Given the auxotrophic nature of pneumococci for certain amino acids, the Ami ABC transporter system, orchestrating oligopeptide uptake, becomes indispensable in host compartments lacking amino acids. The system comprises five exposed Oligopeptide Binding Proteins (OBPs) and four proteins building the ABC transporter channel. Crucially, SBPs determine the specificity of their respective transport systems, thereby governing the range of molecules capable of entering the cell. The five lipoproteins exhibit pairwise sequence identity of ~52–60% and share a very similar overall folding.

AliC was also crystallized in the open conformation, and its structure manifests all the characteristics delineated for AliD. Remarkably, the crystal structure of AliC unveils a distinctive three-dimensional domain-swapped dimer arrangement. In this configuration, the Lobe 1 (comprising Domain I and II) of one monomer becomes intertwined with the Lobe 2 (Domain III) of the adjacent monomer, resulting in an overall architecture that is identical for the two functional monomeric units. The resulting entwined dimer adopts an open conformation, but the width of the ligand-binding cleft is expanded compared to that observed in AliD, measuring 29 Å instead of 16 Å. The observed domain swapping in AliC would be compatible with its insertion into the membrane, given that both N-terminal ends would be oriented toward the same side. Nevertheless, to date, there is no supporting evidence indicating that a domain-swapped dimer represents a functional state of these SBPs, including AliC. The domain swap in AliC results in an extended interface area of 5173.1 Å2 [calculated with PDBe PISA v1.52], occurring at a hinge axis passing through the middle of the loop connecting α7 with β14 (residues 290–294), extending between Lobe 1 and Lobe 2. This loop in AliC contains a glycine residue (G290) that is unique compared to other homologs, which typically have a lysine residue at that position (K287 in AliD). For instance, AliD presents a significant number of aromatic residues decorating the binding-site cavity, promoting the binding oligopeptides with a high hydrophobic residue content. Both AliB and AliC share strongly acidic pockets P3 and P4 but AliC features distinctive basic pockets P1 and P2.

> ASKSEKNADAPKTFSYVYAVDPSSLDYSLTSKSSTSDVIGNVVDGLLENDKYGNLIPSLAEDWSVSKDGLTYTYKLRKGVKWYTSEGEEYAEVKAQDFVTGLKHAADGKSDGLSLVEKSIKGLEAYVSGETNDFSTVGVKALDDYTVEYTLNNPESFWNSKVTTATMLPVNEEFLNATGKDYGAPTPSSILYNGPYFLKSLISKSVIEYEKNPNYWDKENVKIDNVKLTFYDGSDQESLIRSFTQGAYTTARLFPASSNFESTKKEYGDKIVYSPQEATSYYLTVNVNRQSYNKTAKTDESQKTSTKEALLNKNFRQALNFAFNRHAYTAQLNGEEGADKIIRNSLVPDNYVQVAGKTFGQLAQDELLKYGEQWKDVTLTDGKDTIYNPTKAKSAFEKAKSELQAKGVSFPIHLDVPVEQTDVVAVQQTNSLKQSIEETLGTENVIIDVLQMTDNEKESITSQAKVPTQKDYDLNGTGWGPDYQDPATYLNILDAKKGSALKHLGITKGKDPEVVAKVGLDEYKKLLDDAASETSNLDKRYEKYAKAQAWVTDSSLLIPVASSGGSPMVSRTVPFTKAYSQVGIKGDPFIFKGMELQNDIVTTKEYDAAFKKWQKEKLESNAQYQKDLEKHIK> GHMASVTDGKTGVKDASDQNFDYMFKLLIIGNSSVGKTSFLFRYADDTFTPAFVSTVGIDFKVKTVYRHEKRVKLQIWDTAGQERYRTITTAYYRGAMGFILMYDITNEESFNAVQDWATQIKTYSWDNAQVILVGN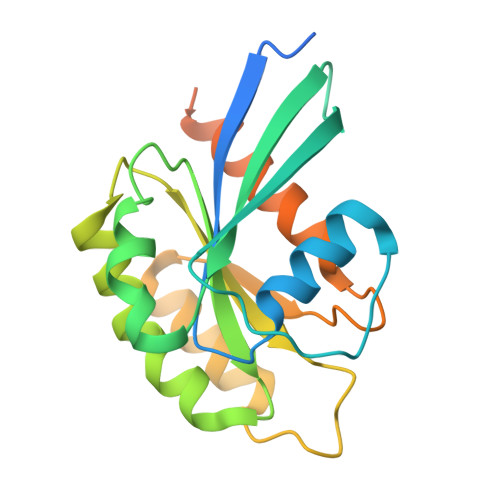KCDMEEERVVPTEKGQLLAEQLGFDFFEASAKENISVRQAFERLVDAICDKMSDSLDTDPSMLGSSKNTRLSDTPPLLQQNCSC>MNIHGFDLGSRYMDLKPLGCGGNGLVFSAVDNDCDKRVAIKKIVLTDPQSVKHALREIKIIRRLDHDNIVKVFEILGPSGSQLTDDVGSLTELNSVYIVQEYMETDLANVLEQGPLLEEHARLFMYQLLRGLKYIHSANVLHRDLKPANLFINTEDLVLKIGDFGLARIMDPHYSHKGHLSEGLVTKWYRSPRLLLSPNNYTKAIDMWAAGCIFAEMLTGKTLFAGAHELEQMQL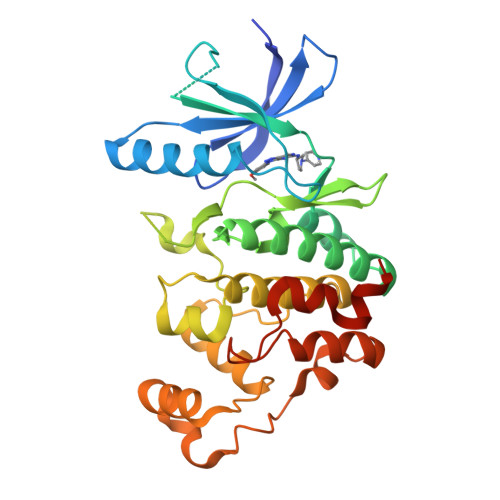ILESIPVVHEEDRQELLSVIPVYIRNDMTEPHKPLTQLLPGISREAVDFLEQILTFSPMDRLTAEEALSHPYMSIYSFPMDEPI[4x]4-amino-6-{[(2-fluorophenyl)methyl]amino}-7-methyl-7H-pyrrolo[2,3-d]pyrimidine-5-carbonitrile 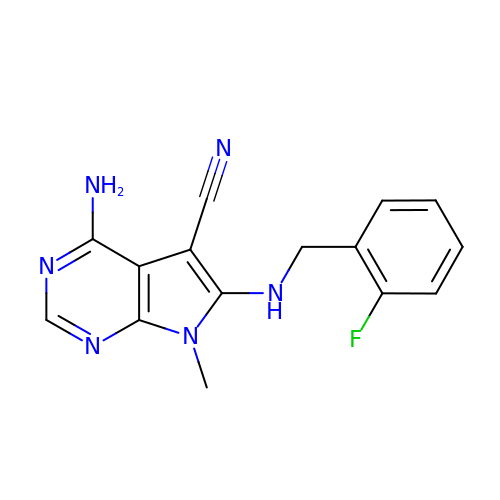| C15 H13 F N6 | BJAJDULYKUREBF-UHFFFAOYSA-N> MKTIIALSYIFCLVFAYPYDVPDYAAAAEPAENSDFYLPGDYLLGGLFSLHANMKGIVHLNFLQVPMCKEYEVKVIGYNLMQAMRFAVEEINNDSSLLPGVLLGYEIVDVCYISNNVQPVLYFLAHEDNLLPIQEDYSNYISRVVAVIGPDNSESVMTVANFLSLFLLPQITYSAISDELRDKVRFPALLRTTPSADHHIEAMVQLMLHFRWNWIIVLVSSDTYGRDNGQLLGERVARRDICIAFQETLPTLQPNQNMTSEERQRLVTIVDKLQQSTARVVVVFSPDLTLYHFFNEVLRQNFTGAVWIASESWAIDPVLHNLTELRHLGTFLGITIQSVPIPGFSEFREWGPQAGPPPLSRTSQSYTCNQECDNCLNATLSFNTILRLSGERVVYSVYSAVYAVAHALHSLLGCDKSTCTKRVVYPWQLLEEIWKVNFTLLDHQIFFDPQGDVALHLEI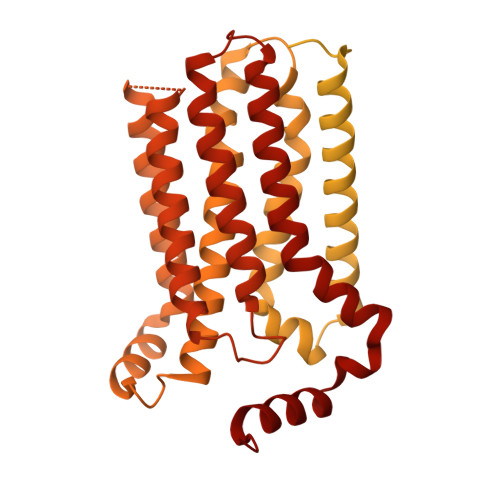VQWQWDRSQNPFQSVASYYPLQRQLKNIQDISWHTINNTIPMSMCSKRCQSGQKKKPVGIHVCCFECIDCLPGTFLNHTEDEYECQACPNNEWSYQSETSCFKRQLVFLEWHEAPTIAVALLAALGFLSTLAILVIFWRHFQTPIVRSAGGPMCFLMLTLLLVAYMVVPVYVGPPKVSTCLCRQALFPLCFTICISCIAVRSFQIVCAFKMASRFPRAYSYWVRYQGPYVSMAFITVLKMVIVVIGMLATGLSPTTRTDPDDPKITIVSCNPNYRNSLLFNTSLDLLLSVVGFSFAYMGKELPTNYNEAKFITLSMTFYFTSSVSLCTFMSAYSGVLVTIVDLLVTVLNLLAISLGYFGPKCYMILFYPERNTPAYFNSMIQGYTMRRD>AGGLSQLVAYGAQDVYLTGNPQITFFKTVYRRYTNFAIESIQQTINGSVGFGNKVSTQISRNGDLITDIVVEFVLTKGGNGGTTYYPAEELLQDVELEIGGQRIDKHYNDWFRTYDALFRMNDDRYNYRRMTDWVNNELVGAQKRFYVPLIFFFNQTPGLALPLIALQYHEVKLYFTLASQVQGVNYNGSSAIAGAAQPTMSVWVDYIFLDTQERTRFAQLPHEYLIEQLQFTGSETATPSATTQASQNIRLNFNHPTKYLAWNFNNPTNYGQYTALANIPGACSGAGTAAATVTTPDYGNTGTYNEQLAVLDSAKIQLNGQDRFATRKGSYFNKVQPYQSIGGVTPAGVYLYSFALKPAGRQPSGTCNFSRIDNATLSLTYKTCSIDA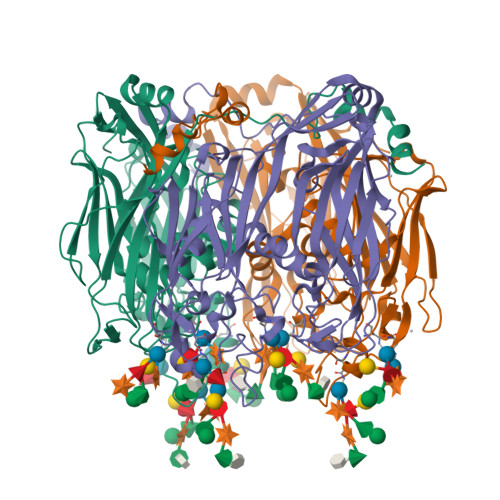TSPAAVLGNTETVTANTATLLTALNIYAKNYNVLRIMSGMGGLAYAN[2x]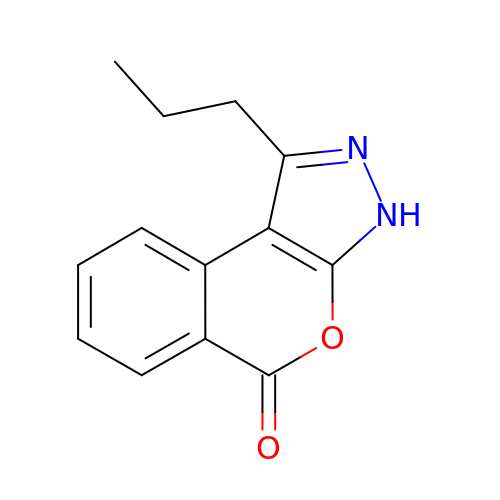1-propylisochromeno[3,4-c]pyrazol-5(3H)-one | C13 H12 N2 O2 | URRDWILHXUGXPV-UHFFFAOYSA-N> VKDLLKFLKAQTKTEEFDAIKIALASPDMIRSWSFGEVKKPETINYRTFKPERDGLFCARIFGPVKDYECLCGKYKRLKHRGVICEKCGVEVTQTKVRRERMGHIELASPTAHIWFLKSLPSRIGLLLDMPLRDIERVLYFESYVVIEGGMTNLERQQILTEEQYLDALEEFGDEFDAKMGAEAIQALLKSMDLEQECEQLREELNETNSETKRKKLTKRIKLLEAFVQSGNKPEWMILTVLPVLPPDLRPLVPLDGGRFATSDLNDLYRRVINRNNRLKRLLDLAAPDIIVRNEKRMLQEAVDALLDNGRRGRAITGSNKRPLKSLADMIKGKQGRFRQNLLGKRVDYSGRSVITVGPYLRLHQCGLPKKMALELFKPFIYGKLELRGLATTIKAAKKMVEREEAVVWDILDEVIREHPVLLNRAPTLHRLGIQAFEPVLIEGKAIQLHPLVCAAYNADFDGDQMAVHVPLTLEAQLEARALMMSTNNILSPANGEPIIVPSQDVVLGLYYMTRDCVNAKGEGMVLTGPKEAERLYRSGLASLHARVKVRITEYEKDANGELVAKTSLKDTTVGRAILWMIVPKGLPYSIVNQALGKKAISKMLNTCYRILGLKPTVIFADQIMYTGFAYAARSGASVGIDDMVIPEKKHEIISEAEAEVAEIQEQFQSGLVTAGERYNKVIDIWAAANDRVSKAMMDNLQTETVINRDGQEEKQVSFNSIYMMADSGARGSAAQIRQLAGMRGLMAKPDGSIIETPITANFREGLNVLQYFISTHGARKGLADTALKTANSGYLTRRLVDVAQDLVVTE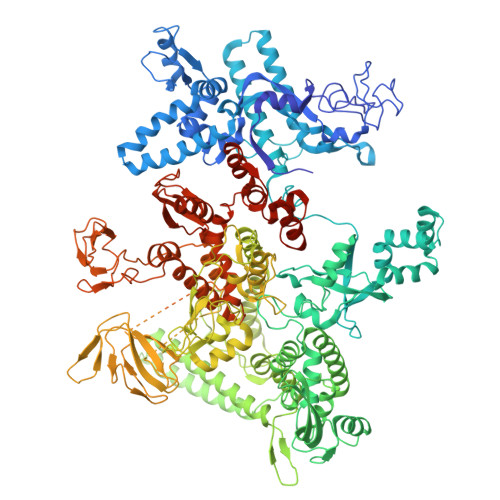DDCGTHEGIMMTPVIEGGDVKEPLRDRVLGRVTAEDVLKPGTADILVPRNTLLHEQWCDLLEENSVDAVKVRSVVSCDTDFGVCAHCYGRDLARGHIINKGEAIGVIAAQSIGEPGTQLTMRTFHIGGAASRAAAESSIQVKNKGSIKLSNVKSVVNSSGKLVITSRNTELKLIDEFGRTKESYKVPYGAVLAKGDGEQVAGGETVANWDPHTMPVITEVSGFVRFTDMIDGQTITRQTDELTGLSSLVVLDSAERTAGGKDLRPALKIVDAQGNDVLIPGTDMPAQYFLPGKAIVQLEDGVQISSGDTLARIPQESGGTKDITGGLPRVADLFEARRPKEPAILAEISGIVSFGKETKGKRRLVITPVDGSDPYEEMIPKWRQLNVFEGERVERGDVISDGPEAPHDILRLRGVHAVTRYIVNEVQDVYRLQGVKINDKHIEVIVRQMLRKATIVNAGSSDFLEGEQVEYSRVKIANRELEANGKVGATYSRDLLGITKASLATESFISAASFQETTRVLTEAAVAGKRDELRGLKENVIVGRLIPAGTGYAYHQDRMRRRAAGEAPAAPQVTAEDASASLAELLNAGLGGSDNELE> 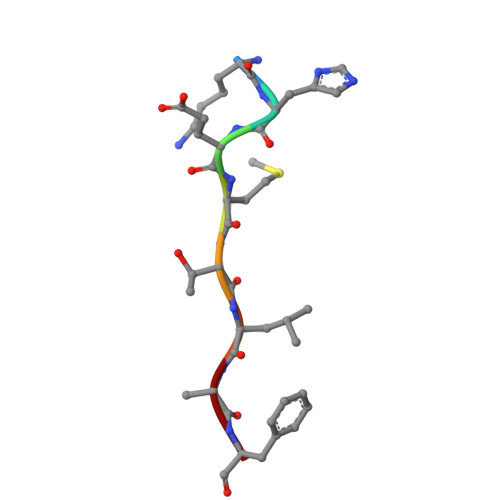KHEMTLKF> TSKATIRDLNDPSQVKTLQEKASKGAGTVVAVIDAGFDKNHEAWRLTDKTKARYQSKEDLEKAKKEHGITYGEWVNDKVAYYHDYSKDGKTAVDQEHGTHVSGILSGNAPSETKEPYRLEGAMPEAQLLLMRVEIVNGLADYARNYAQAIRDAVNLGAKVINMSFGNAALAYANLPDETKKAFDYAKSKGVSIVTSAGNDSSFGGKTRLPLADHPDYGVVGTPAAADSTLTVASYSPDKQLTETATVKTDDHQAKEMPVLSTNRFEPNKAYDYAYANRGMKEDDFKDVKGKIALIERGDIDFKDKIANAKKAGAVGVLIYDNQDKGFPIELPNVDQMPAAFISRKDGLLLKDNSKKTITFNATPKVLPTASDTKLSRFSSWGLTADGNIKPDIAAPGQDILSSVANNKYAKLSGTSMSAPLVAGIMGLLQKQYETQYPDMTPSERLDLAKKVLMSSATALYDEDEKAYFSPRQQGAGAVDAKKASAATMYVTDKDNTSSKVHLNNVSDKFEVTVTVHNKSDKPQELYYQATVQTDKVDGKHFALAPKALYETSWQKITIPANSSKQVTVPIDASRFSKDLLAQMKNGYFLEGFVRFKQDPKKEELMSIPYIGFRGDFGNLSALEKPIYDSKDGSSYYHEANSDAKDQLDGDGLQFYALKNNFTALTTESNPWTIIKAVKEGVENIEDIESSEITETIFAGTFAKQDDDSHYYIHRHANGKPYAAISPNGDGNRDYVQFQ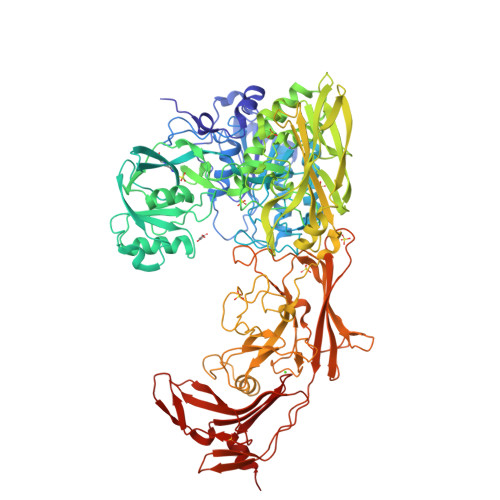GTFLRNAKNLVAEVLDKEGNVVWTSEVTEQVVKNYNNDLASTLGSTRFEKTRWDGKDKDGKVVVNGTYTYRVRYTPISSGAKEQHTDFDVIVDNTTPEVATSATFSTEDRRLTLASKPKTSQPIYRERIAYTYMDEDLPTTEYISPNEDGTFTLPEEAETMEGGTVPLKMSDFTYVVEDMAGNITYTPVTKLLEGHS> GSMVENSELRKAGLKVTLPRVKILQMLDSAEQRHMSAEDVYKALMEAGEDVGLA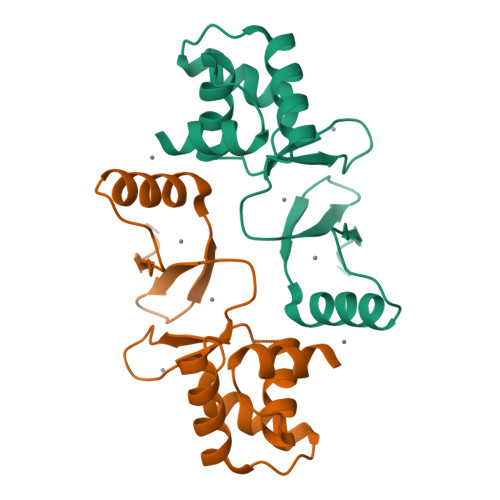TVYRVLTQFEAAGLVVRHNFDGGHAVFELADSGHHDHMVCVDTGEVIEFMDAEIEKRQKEIVRERGFELVDHNLVLYVRKKK>GTGSRPITDVVFVGAARTPIGSFRSAFNNVPVTVLGREALKGALKNANVKPSLVQEAFIGVVVPSNAGQGPARQVVLGAGCDVSTVVTAVNKMCASGMKAIACAASILQLDLQEMVVAGGMESMSCVPFYLPRGEIPFGGTKLIDGIPRDGLNDVYNDILMGACADKVAKQFAITREEQDKYAILSYKRSAAAWKEGIFAKEIIPLEVTQGKKTITVEEDEEYKKVNFEKIPKLKPAFTSEGSVTAANASTLNDGAAMVVMTTVDGAKKHGLKPLARM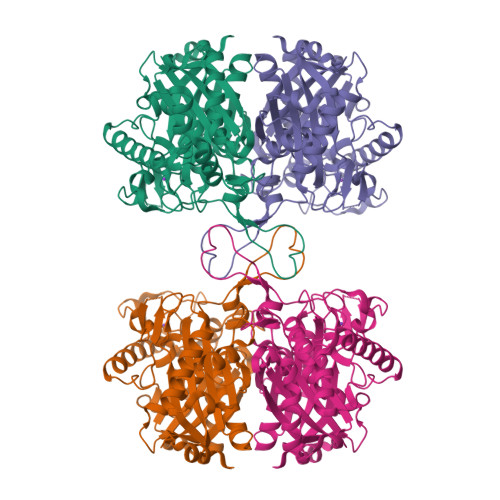LAYGDAATHPIDFGIAPASVIPKVLKLAGLQIKDIDLWEINEAFAVVPLYTMKTLGLDESKVNIHGGAVSLGHPIGMSGARIVGHLVHTLKPGQKGCAAICNGGGGAGGMIIEKL[2x]> MSLPAHLQQTFSPEEIQFIVENEPIKIFPRITTRQKIRGDDRGTGNHTRWQLITTDDKALNNMVAMRSTEVVLWIALLLKQQSKCSIVAPQWLTTKELDRKIQYEKTHPDRFSELP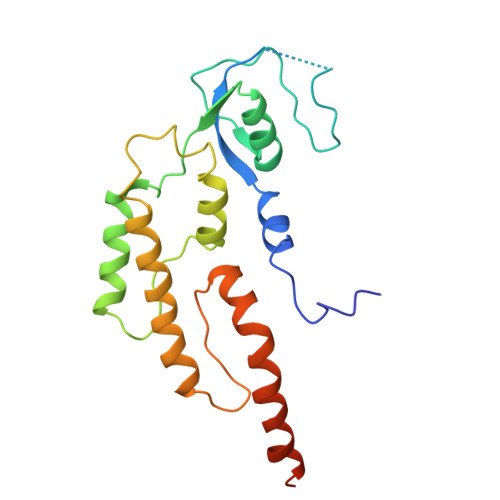WNWLVLARILFNKAKDDFHDPIHELRGKIQDLREIRQIKVLKGLKYLNESHLQLDNLSLLEINELRPFITEIMDKLREIHTASLTAGTENDEEEFNI ALPHA-DIFLUOROMETHYLORNITHINE | C6 H12 F2 N2 O2 | 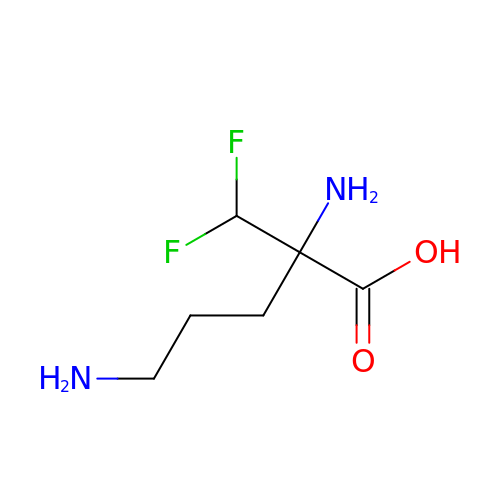VLCYCQAOQCDTCN-ZCFIWIBFSA-N> DLDTHFTQYKLARPYIADCPNCGHSRCDSPIAIEEVRGDAHAGVIRIQTSAMFGLKTDGVDLAYMSFMNGKTQKSIKIDNLHVRTSAPCSLVSHHGYYILAQCPPGDTVTVGFHDGPNRHTCTVAHKVEFRPVGREKYRHPPEHGVELPCNRYTHKRADQGHYVEMHQPGLVADHSLLSIHSAKVKITVPSGAQVKYYCKCPDVREGITSSDHTTT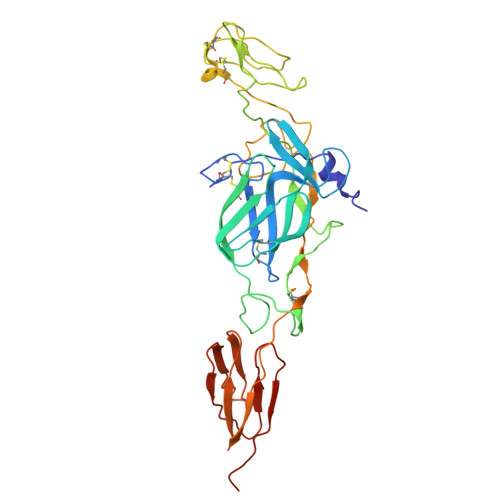CTDVKQCRAYLIDNKKWVYNSGRLPRGEGDTFKGKLHVPFVPVKAKCIATLAPEPLVEHKHRTLILHLHPDHPTLLTTRSLGSDANPTRQWIERPTTVNFTVTGEGLEYTWGNHPPKRVWAQESGE>[2x]MLCEIECRALSTAHTRLIHDFEPRDALTYLEGKNIFTEDHSELISKMSTRLERIANFLRIYRRQASELGPLIDFFNYNNQSHLADFLEDYIDFAINEPDLLRPVVIAPQFSRQMLDRKLLLGNVPKQMTCYIREYHVDRVIKKLDEMCDLDSFFLFLHGRAGSGKSVIASQALSKSDQLIGINYDSIVWLKDSGTAPKSTFDLFTDILLMLKSEDDLLNFPSVEHVTSVVLKRMICNALIDRPNTLFVFDDVVQEETIRWAQELRLRCLVTTRDVEISNAASQTCEFIEVTSLEIDECYDFLEAY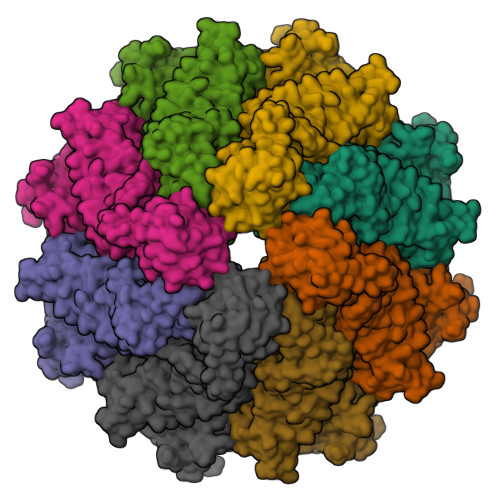GMPMPVGEKEEDVLNKTIELSSGNPATLMMFFKSCEPKTFEKMAQLNNKLESRGLVGVECITPYSYKSLAMALQRCVEVLSDEDRSALAFAVVMPPGVDIPVKLWSCVIPVDICSNEEEQLDDEVADRLKRLSKRGALLSGKRMPVLTFKIDHIIHMFLKHVVDAQTIANGISILEQRLLEIGNNNVSVPERHIPSHFQKFRRSSASEMYPKTTEETVIRPEDFPKFMQLHQKFYDSLKNFACC>[4x]MELLQGKTFVVMGVANQRSIAWGIARSLHNAGAKLIFTYAGERLERNVRELADTLEGQESLVLPCDVTNDEELTACFETI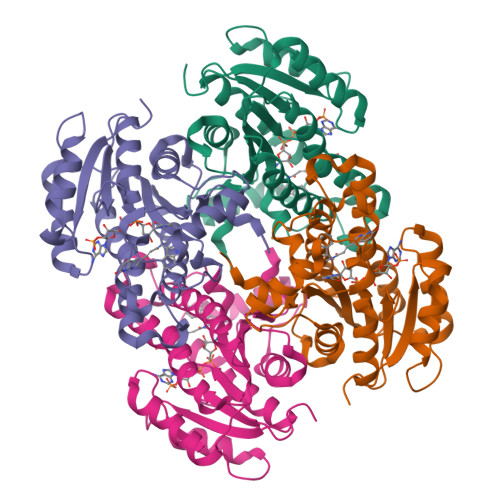KQEVGTIHGVAHCIAFANRDDLKGEFVDTSRDGFLLAQNISAFSLTAVAREAKKVMTEGGNILTLTYLGGERVVKNYNVMGVAKASLEASVKYLANDLGQHGIRVNAISAGPIRTLSAKGVGDFNSILREIEERAPLRRTTTQEEVGDTAVFLFSDLARGVTGENIHVDSGYHILGL> MASWSHPQFE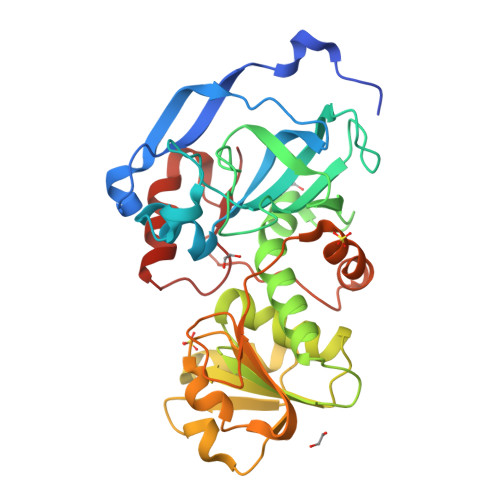KGAAAPSESIPSVNKAWVYSEYGKTSDVLKFDPSVAVPEIKEDQVLIKVVAASLNPVDFKRALGYFKDTDSPLPTIPGYDVAGVVVKVGSQVTKFKVGDEVYGDLNETALVNPTRFGSLAEYTAADERVLAHKPKNLSFIEAASLPLAIETAHEGLERAELSAGKSVLVLGGAGGVGTHIIQLAKHVFGASKVAATASTKKLDLLRTLGADLAIDYTKENFEDLPEKFDVVYDAVGETDKAVKAVKEGGKVVTIVGPATPPAILFVLTSKGSVLEKLKPYLESGKVKPVLDPTSPYPFTKVVEAFGYLESSRATGKVVVYPI> SKNEWRKSAIANTLLYLRLKNIYVSADDFVEEQNVYVLPKNLLKKFIEISDVKIQVAAFIYGMSAKDHPKVKEIKTVVLVPQLGHVGSVQISNIPDIGDLPDTEGLELLGWIHTQTEELKFMAASEVATHSKLFADKKRDCIDISIFSTPGSVSLSAYNLTDEGYQWGEENKDIMNVLSEGFEPTFSTHAQLLLSDRITGNFIIPSGNVWNYTF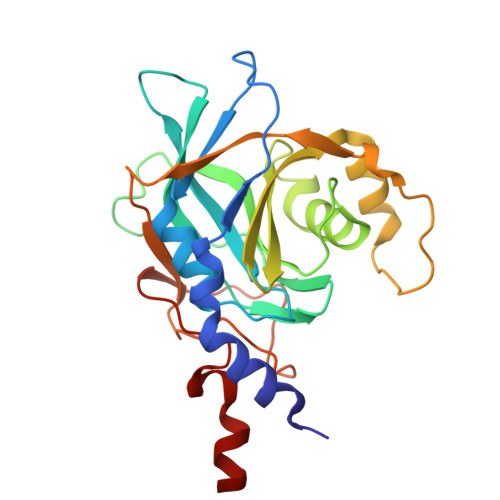MGTAFNQEGDYNFKYGIPLEFYNEMHRPVHFLQF FliG forms a ring on the cytoplasmic face of the MS ring. directly involved in the switching of the flagellar motor. generation and in stator assembly around the rotor.

deletion at positions 169 to 171. deletion, indicating that the motor is locked in the CW state. to the one introduced by the in-frame PAA deletion. is different from that of Tm-FliGMC. is also different in these two structures. here, we propose a new model for arrangement of FliG subunits in the motor. interaction between helix E and FliGM of the neighbor. the orientation of the neighboring FliGM domain. orientation of FliGCC to cause anomalous switching behavior. change in the interaction between FliGCC and MotA.

> QVKPFSFVRDTDPVQLVNFLQSEHPQTIAVVLSYLDPPVAAQILGALPEELQTEVLKRIALLERTSVKEIERNLEKKISGFVSRTFSKVGGIDTAAEIMNNLDRTTEKKIMDKLVQENPELADEIRRRMFVFEDILKLDDRSIQLVLREVDTRDLALALKGASDELKEKIFKNMSKRAAALLKDELEYMGPVRLKDVEEAQQKIINIIRRLEEAGEIVIARGGGEELIM> PGGVPWIAVGDETSVTSPGALRRMTSKDIPETAIINTDNSSGAVPSESALVPYIDEPLVVVTEHAITNFTKAEMALEFNREFLDKMRVLSVSPKYSDLLTYVDCYVGVS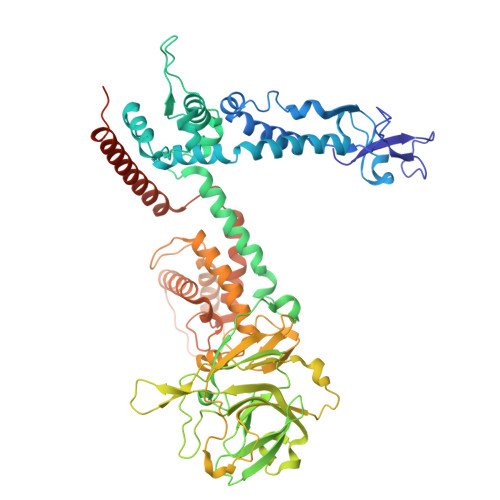ARQALNNFQKQVPVITPTRQTMYVDSIQAALKALEKWEIDLRVAQTLLPTNVPIGEVSCPMQSVVKLLDDQLPDDSLIRRYPKEAAVALAKRNGGIQWMDVSEGTVMNEAVNAVAASALAPSASAPPLEEKSKLTEQAMDLVTAAEPEIIASLVPVPAPVFAIPPKPADYNVRTLRIDEATWLRMIPKSMNTPFQIQVTDNTGTNWHLNLRGGTRVVNLDQIAPMRFVLDLGGKSYKETSWDPNGKKVGFIVFQSKIPFELWTAASQIGQATVVNYVQLYAEDSSFTAQSIIATTSLAYNYEPEQLNKTDPEMNYYLLATFIDSAAITPTNMTQPDVWDALLTMSPLSAGEVTVKGAVVSEVVPADLIGSYTPESLNTSLPNDAARCMIDRASKIAEAIKIDDDAGPDEYSPNSVPIQGQLAISQLETGYGVRIFNPKGILSKIASRAMQAFIGDPSTIITQAAPVLSDKNNWIALAQGVKTSLRTKSLSAGVKTAVSKLSSSESIQNWTQGFLDKVSAHFPAPKPDCPTSGDSGESSNRRVKRDSYAGVVKRGYTR>MRGSHHHHHHGSMTDHVREADDANIDDLLGDLGGTARAERAKLVEWLLEQGITPDEIRATNPPLLLATRHLVGDDGTYVSAREISENYGVDLELLQRVQRAVGLARVDDPDAVVHMRADGEAAARAQRFVELGLNPDQVVLVVRVLAEGLSHAAEAMRYTALEAIMRPGATELDIAKG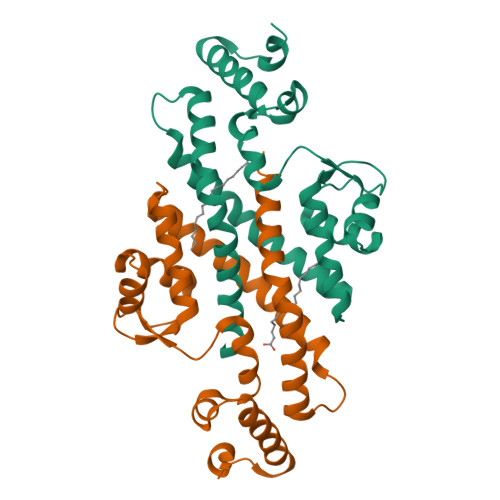SQALVSQIVPLLGPMIQDMLFMQLRHMMETEAVNAGERAAGSSP[2x]> MTVEQMMKSGEMIRSVCLGKTKVAEELVNGLRESKFADVKELKC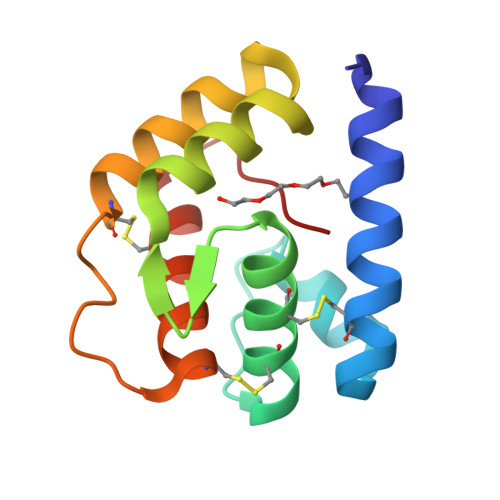YVNCVMEMMQTMKKGKLNYDASVKQIDTIMPDELAGPMRAALDICRTVADGIKNNCDAAYVLLQCLSKNNPKFIFP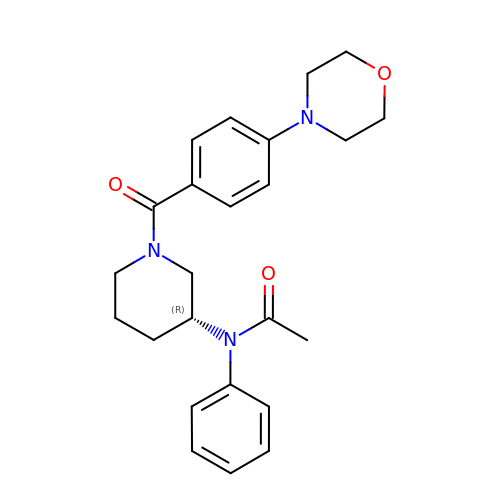N-{(3R)-1-[4-(morpholin-4-yl)benzene-1-carbonyl]piperidin-3-yl}-N-phenylacetamide | C24 H29 N3 O3 | ZPBAECMYHZRSTO-HSZRJFAPSA-N2-(1,3-benzoxazol-2-ylamino)spiro[1,6,7,8-tetrahydroquinazoline-4,1'-cyclopentane]-5-one 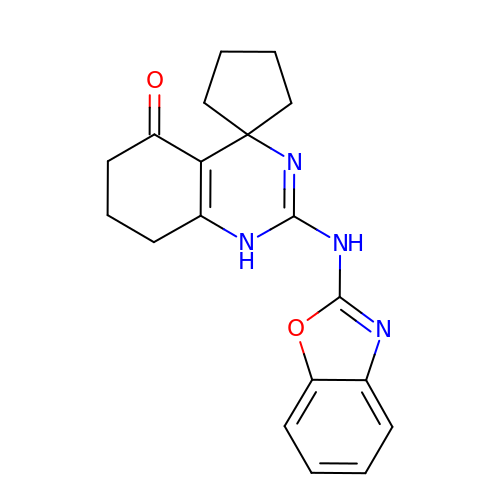| C19 H20 N4 O2 | FDNVTCDQGOVLPM-UHFFFAOYSA-N4-[[(R)-(5-ethoxy-2-fluoranyl-3-propan-2-yloxy-phenyl)-(4-phenyl-1H-imidazol-2-yl)methyl]amino]benzenecarboximidamide 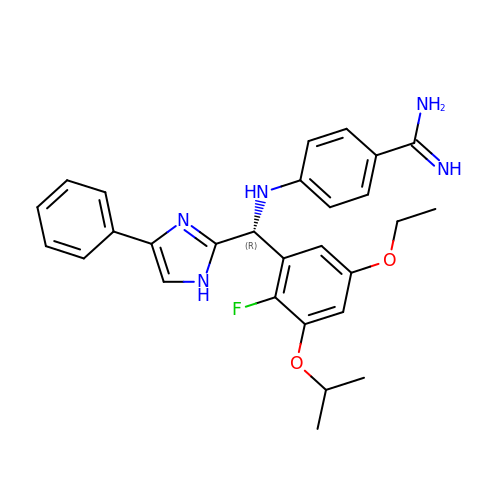| C28 H30 F N5 O2 | FEJKACPKVXNBAK-AREMUKBSSA-N>[2x]QRCGSQGGGA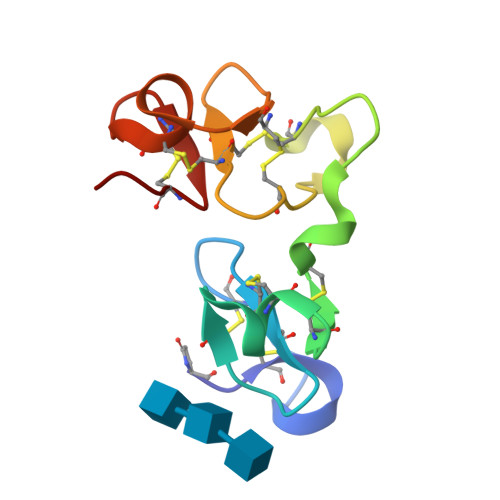TCPGLRCCSIWGWCGDSEPYCGRTCENKCWSGERSDHRCGAAVGNPPCGQDRCCSVHGWCGGGNDYCSGGKCQYRCSSS>MIALAVSGALLSSMTPAVAQPQNPDDAAIAQAEENVSAGDGEVARLAGSLSSTDAEINRVELEMGALREEVNKSLVDLHDAQAIAEQARQDALAAKKDLDDSQAQIEAAQERLDEISRAAYRQNGTSKGLSGISGNGNSEDALDRQTYLRTSAEKQQAAVEELDRLRTENANKESVLRQARIVAEQREAEAVEKQVQTEAAIAANSEQLNVLTNNRSTLVAQRDGAERNLAIARAQADNLQGQRAEYEEFQQAEQARIQAEAEAQAAAEEKRRADEAAAQAAAEAQEAAQQAQAAEEAQAAQAAETAQAQAAQAAETQAAQAAQAQAEANDRAAAQQRAAEAQAAAEQAQREADAQAANDAQAQALREQALTAASIAAAALIAASQSSHATTQNPYPTDEDADPTDIADIQGPTQPGTGESGDSQSNSSDNDSTGNDSTGSDSSDSDSSGNDSSEVISGDRSAQIETVIARAMSQLGVQYAWGGGNANGPTLGIRDGGVADSYGDYNKVGFDCSGLTLYAFAGVGISLPHYTGYQYQHGTKVSPSEMQRGDLIFYGPGASQHVAIYLGDGQMIEAPNSGSVVKISPVRWSGMTESVVRLI[2x]

In the order Corynebacteriales, which includes the important pathogens Mycobacterium tuberculosis and Corynebacterium diphtheriae, the most important murein hydrolase for cell separation is the endopeptidase RipA. We present here the crystal structure of a full-length RipA homologue from Corynebacterium glutamicum, Cg1735, which reveals an unusual mode of autoinhibition. We describe how this autoinhibition is relieved by the conserved transmembrane protein Cg1604 and propose an FtsEX-independent model for septal control of PG hydrolysis via the Cg1604–Cg1735 complex. In this model, two septal TM proteins, Cg1603, with a cytoplasmic N-terminal globular core, and Cg1604, with a C-terminal globular core exposed to the cell envelope, form a signaling complex that couples intracellular cell division events with PG hydrolysis during the last stages of cell separation.

The full periplasmic region of Cg1735 (residues 20 to 600) was crystallized in two different crystal forms with a high (80 to 85%) solvent content. The trigonal form was solved by single-wavelength anomalous diffraction (SAD) techniques at 3.5 Å resolution and the orthorhombic form by molecular replacement at 4.5 Å resolution. Both structures reveal a tight complex between the C-terminal NlpC/P60 CD (residues 460 to 600) and an anti-parallel two-helical coiled-coil domain (CC1, residues 46 to 238) corresponding to the highly conserved N-terminal region in the RipA family. In the orthorhombic crystal form, the long interconnecting linker (residues 239 to 372) is present but disordered in the crystal. Instead, crystal contacts in the trigonal form promote a disorder-to-order transition in this region that extends the short HL helix into a full anti-parallel two-helical coiled-coil domain, CC2 (residues 243 to 386). The presence of this new structural element precludes complex formation between the CD and the CC1 domain to occur within the same monomer. Instead, the CD–CC1 complex now forms between two different monomers in the asymmetric unit. Analytical ultracentrifugation experiments at different protein concentrations showed that full-length RipA behaves as a monomer in solution, with no trace of dimer formation even at 5 mg/mL, the highest tested concentration, demonstrating that dimerization is due to crystallization-induced domain-swapping effects. The CC2 domain is deeply engaged in—and stabilized by—crystal packing contacts in the trigonal space group. The structure of trigonal Cg1735 soaked in Cl4K2Pt was determined by SAD phasing: two major and several minor Pt sites in the asymmetric unit were found with SHELXD, and the experimental phases obtained with PHASER were significantly improved by density modification with PARROT from the CCP4 suite, as the crystal has a high (85%) solvent content.>[5x]GAMNECAFGTKDPVYLNYHDHVWGQPLYDSKALFK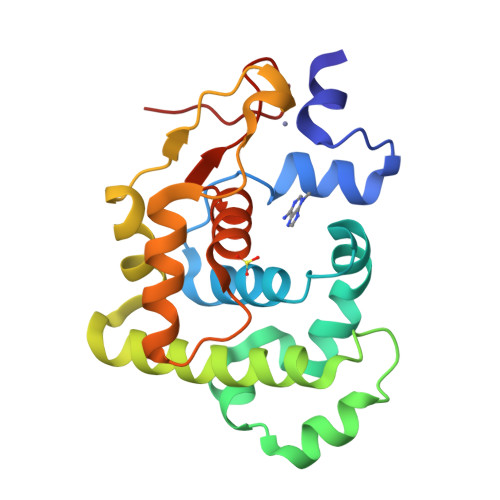LLALESQHAGLSWLTILKKKEAYEEAFYDFEPEKVAQMTAQDIDRLMTFPNIVHHRKKLEAIVNQAQGYLKIEQAYGSFSKFLWSYVNGKPKDLQYEHASDRITVDDTATQLSKDLKQYGFKFLGPVTVFSFLEAAGLYDAHLKDCPSKPKHN>GGSKVQQYRLDELAHLVKGELIGEGSLQFSNLASLENAEVNHLTFVNGEKHLDQAKVSRAGAYIVTAALKEHLPEKDNFIIVDNPYLAFAILTHVFDKKISSTGIESTARIHPSAVISETAYIGHYVVIGENCVVGDNTVIQSHTKLDDNVEVGKDCFIDSYVTITGSSKLRDRVRIHSSTVIGGEGFGFAPYQGKWHRIAQLGSVLIGNDVRIGSNCSIDRGALDNTILEDGVIIDNLVQIAHNVHIGSNTAIAAKCGIAGSTKIGKNCILAGACGVAGHLSIADNVTLTGMSMVTKNISEAGTYSSGTGLFENN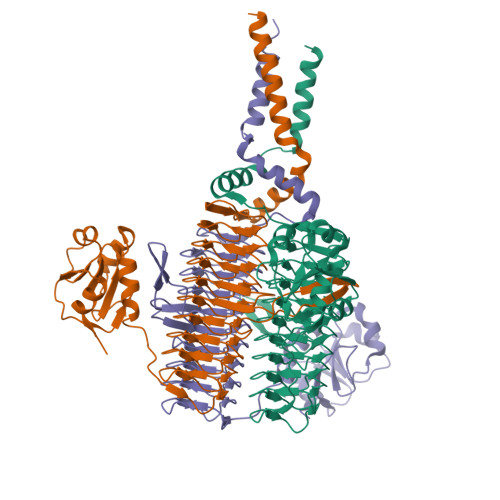HWKKTIVRLRQLADVPLTQITKRLDHIQAQIESLESTFNLR[3x]>[2x]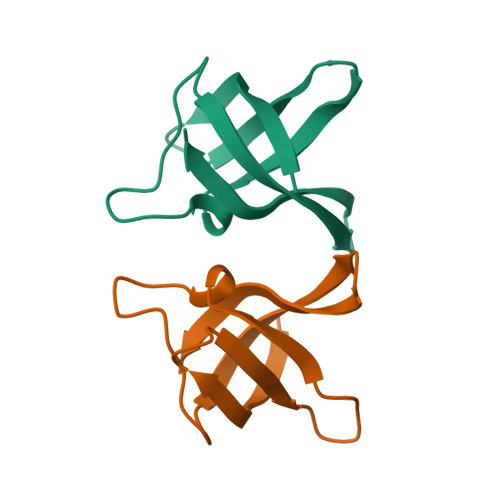MQEGKVKWFNNEKGYGFIEVEGGSDVFVHFTAIQGEGFKTLEEGQEVSFEIVQGNRGPQAANVVKL> MFRMPRPIRAT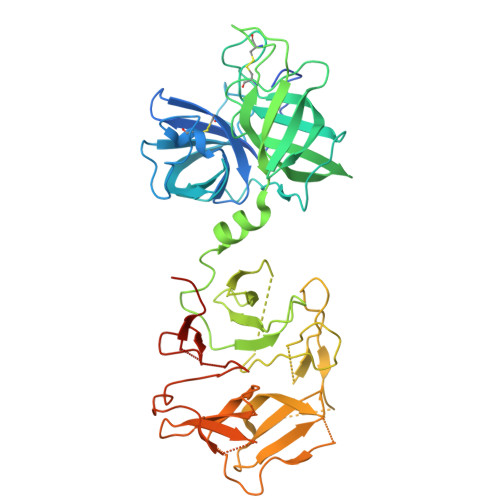ALSAAVLAGALASTPAQATVGDPTTDAKLDFTARLTIGTDYRSCSGALVDTQWVLTAASCFADDPNQPDTVAAGKPAQLTRATVGRADSNIANGYVREVVELVPHPERDMVLARLDKAIPDIAPVRLASDAPTAGTPLTAVGFGRTKDEWVPIQRHQGAFTVTSVTAGAVNVTGQGGDAICAGDTGGPLLQDKNGTLHLVGVNNRSMQGGCYGSETTSTDAIAAMSDADFVTQTVNRDLGTGNLSDLVASADFNSDGRTDVAAVLEDGSLHAFYAKPDGTLEYGRELWNDNTWSPMVQIIGGDFNSDGNGDIAAVRSDGTLNLYTGTATGILNKSKPMWHDTSWKTIKQVTRFKFNGRDGLVAQWGDGNLYGYYTGTDGTLTGTKVKMWPDATWGKTRLTGTADINADGRDDLTAVRDDGSLNWYAGNTKGGLDAARKLWPDNTWTPMKRIIGGDFNGDNKGDIAAVGGQSTLLLYTGTGTGTLNKGIAMRPASGSHHHHHHHH7-[6-(3-HYDROPEROXY-OCT-1-ENYL)-2,3-DIOXA-BICYCLO[2.2.1]HEPT-5-YL]-HEPT-5-ENOIC 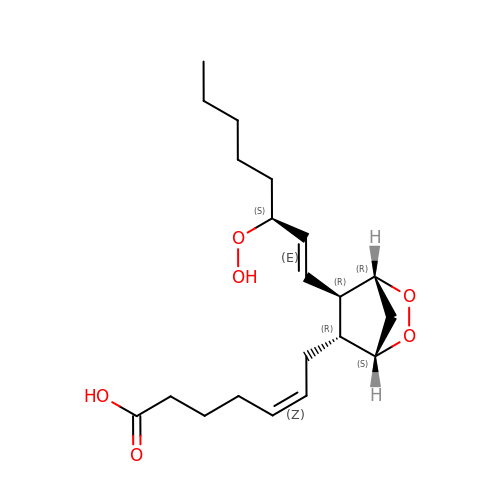ACID | C20 H32 O6 | SGUKUZOVHSFKPH-YNNPMVKQSA-N(R)-IBUPROFENOYL-COENZYME A | C34 H53 N7 O17 P3 S | 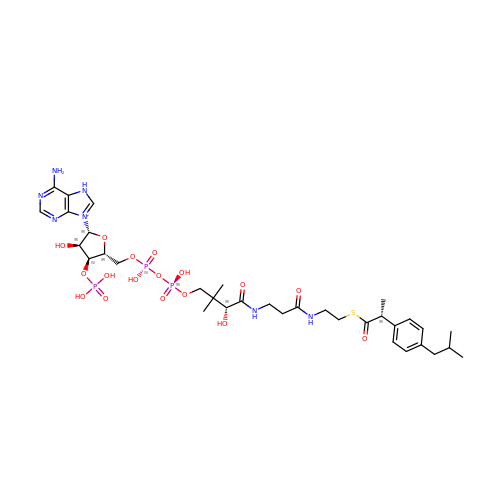NXIKDQUQQHUCJH-NGSKWOHTSA-O>AAVIEKRATCSNGKTVGDASCCAWFDVLDDIQQNLFHGGQCGAEAHESIRLVFHDCIAISPAMEAQGKFGGGGCDGSIMIFDDIETAFHPNIGLDEIVKLQKPFVQKHGVTPGDFIAFAGAVALSNCPGAPQMNFFTGRAPATQPAPDGLVPEPFHTVDQIINRVNDAGEFDELELVWMLSAHSVAAVNDVDPTVQGLPFDSTPGIFDSQFFVETQLRGTAFPG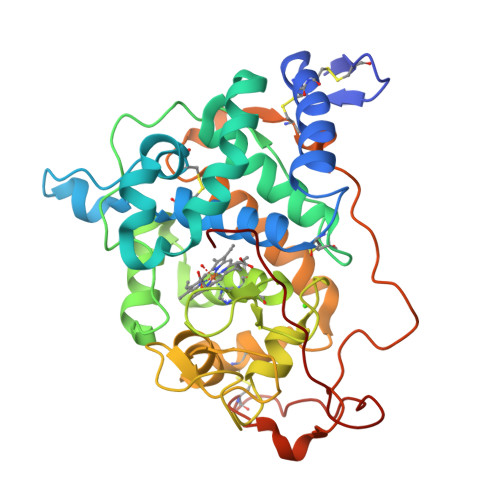SGGNQGEVESPLPGEIRIQSDETIARDSRTACEWQSFVNNQSKLVDDFQFIFLALTQLGQDPNAMTDCSDVIPQSKPIPGNLPFSFFPAGKTIKDVEQACAETPFPTLTTLPGPETSVQRIPPPPGA[2x]> MFYSEAILSKKGPLAKVWLAAHWEKKLSKVQTLHTSIEQSVHAIVTEETAPMALRLSGQLMLGVVRIYSRKARYLLEDCTEALMRLKMSFQPGQVDMIEPATALQSLKGKDAVTQSANLTLPETITEFDLLVPDSTFDFQWSQLLRTPSRSSNTLELHSLPISSSPSFPSSQLSIEAGRNAQVESGFSLGESFAHVGNDMQFHLPISNSGAATPRSVHSDNQSQISIEVGRDAPAAAATDLSGIIGPQMTKSPASSVTHFSTPSMLPIGGTSLDDELLAPVDDLNLDLGLDDLLGDEQGANAPAIEADEQAETSSIHLPSDIMEDDSSRPAAAGVEEGQVVESATAPQQEKINPQKTVRRQRAIIDPVTELSSKQMKKQLADTSSITSPLCLNTSSIVFNATVNFTRNGKFNTSIFSSNLNPKVNELLQADFKQAILRKRKNESPEEVEPAKHQRTDTSTENQETAEVLDPEEIAAAELANITEAAIATLPQETVVQPEGEAP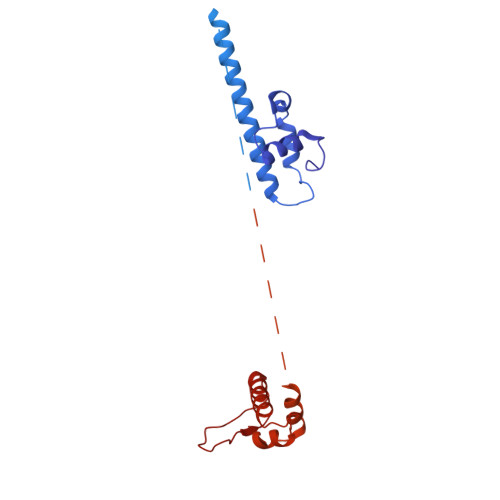ELGSPMGFPVTALESADDSLFDAPPVMLDEADLLGSERLDSSVSEALPSSQTAKDSLRNKWDPYTEGEKVSFQTLSAGCNREEAVQLFFDVLVLATKDVISVKQDVAIQNEITLTAKRGMLLSSL> ATFEIVNRCSYTVWAAASKGDAALDAGGRQLNSGESWTINVEPGTNGGKIWARTDCYFDDSGSGICKTGDCGGLLRCKRFGRPPTTLAEFSLNQYGKDYIDISNIKGFNVPMNFSPTTRGCRGVRCAADIVGQCPAKLKAPGGGCNDACTVFQTSEYCCTTGKCGPTEYSRFFKRLCPDAFSYVLDKPT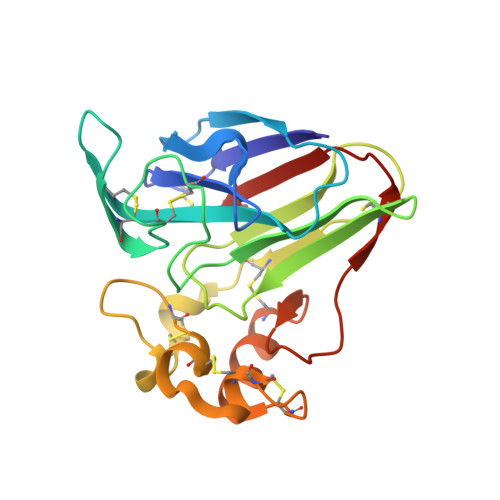TVTCPGSSNYRVTFCPT>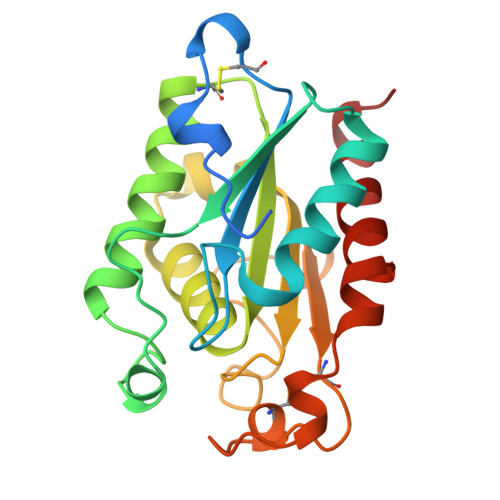 LPTSNPAQELEARQLERTTRDDLINGNSASCADVIFIYARGSTETGNLGTLGPSIASNLESAFGKDGVWIQGVGGAYRATLGDNALPRGTSSAAIREMLGLFQQANTKCPDATLIAGGHSQGAALAAASIEDLDSAIRDKIAGTVLFGYTKNLQNRGRIPNYPADRTKVFCNTGDLVCTGSLIVAAPHLAYGPDARGPAPEFLIEKVRAVRGSA> MASLPAPPTPLGSCPRGRGGGRVVARPRRAGLACAARSCYRFRTDDDGVVDVAVSGEDGDGGGGGYAVSVEVPGTRGREGGLVLRASGSGEGVPLAPAAGGASLAAELSFDPTRAP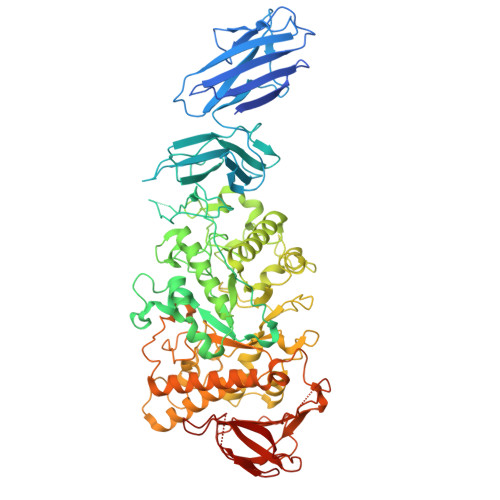FYLSFLLTDASGAEIRTHRKTSFRVPVGVGPGSPAPLGMSISGDGAVNFAVYSKNANAVSLYLYAAAVGGGGGDEPALEIDLDPYIHRTGNVWHVSLASVDGYVSYAFCCGGIRRPLLDPYAKVIGDFVSSNSVYDEGVTAPSMRCFASLAIAPSYNWGRDRHPRLPLEKLVVYRANVALFTKDRSSGLPDDAAGTFTGLSAKVEHFRSLGVNAILLEPVFPFHQVKGPYFPYHFFSPMNLYSSKGLSVSAIKSMKDMVRVMHRNGIEVLLEVVFTHTAEGESECQTISMRGIDNSSYYIANGIAGCKASILNCNHPVTQKLILDSLRHWVLDFHVDGFCFINAPFLVRGPGGEYLSRPPLLEAITFDPVLSMTKIIADPWSPLDISNVQFPFPHWKRWAEVNTRFSIDVRKFLKREALISDLATRLCGSGDLFSTRGPAFSFNHVSRNSGLSLVDLVSFSNDDLLSESSWNCGEEGPSENSAVLQTRLRQIRNFLFILFVSLGVPVLNMGDECGHSAAGSVSYKDRGPLNWRGMKTTFVKEVTGFISFLTALRSRRGDIFQRREFLKLENIHWYGSDLCEPGWDDPTSNFLCMHINAEVDEMAADSVRGDLYICFNANEESVSAALPALAEGSVWLRLVDTSLAFPGFFATESNPKVQQVPGLSSYHVEAHTCVLFESKSALA>GSHMPGPVARLAPQAVLTPPSAASLFLVLVAGDSDDDRATVCDVISGIDGPLKAVGFRELAGSLSCVVGVGAQFWDRVSASSKPAHLHPFVPLSGPVHSAPSTPGDLLFHIKAARKDLCFELGRQIVSALGSAATVVDEVHGFRYFDSRDLLGFVDGTEN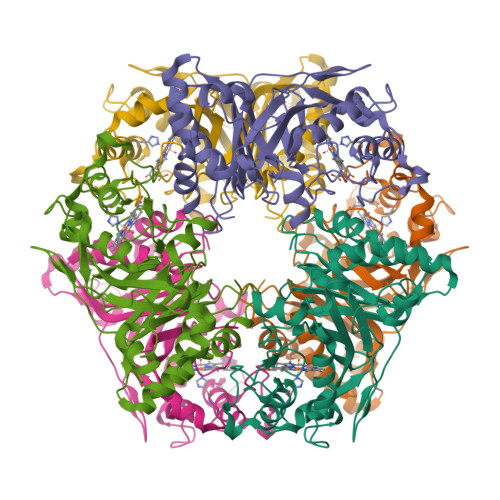PTDDDAADSALIGDEDPDFRGGSYVIVQKYLHDMSAWNTLSTEEQERVIGRTKLENVELDDDAQPSNSHVTLNTIVDDDGVEHDILRDHMAFGSLGEAEYGTYFIGYAKDPAVTELMLRRMFLGEPPGNYDRVLDFSTAATGTLFFVPSRDVLESLGDEPAGAESAPEDPVEPAAAGPYDLSLKIGGLKGVSQ[3x]> GETARLLRAPVAGTIKLGKKARTRPYRTRHGEEALLAEANFDLVLEGKGRKETFAILQGSTIFVQDGDKVAAEAILAEV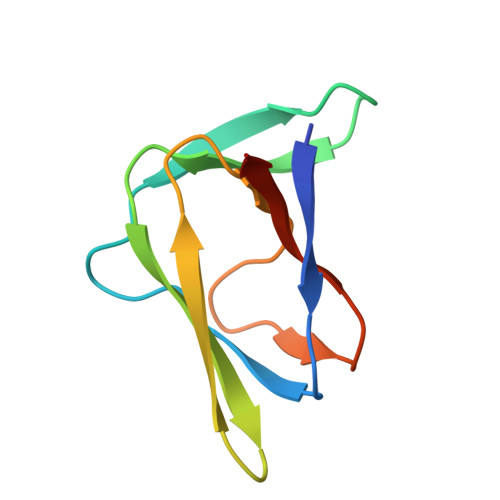PVSGR>[2x]GGGTPKAPNLEPPLPEEEKEGSDLRPVVIDGSNVAMSHGNKEVF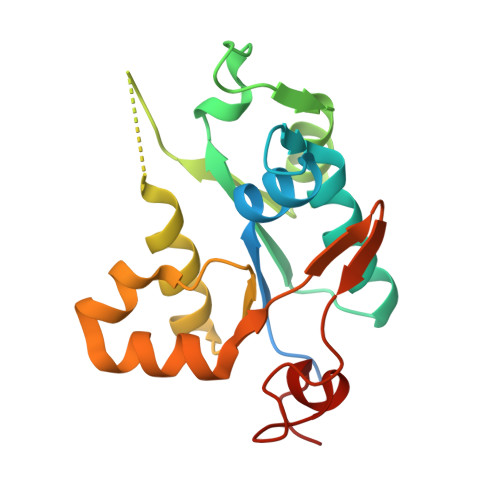SCRGILLAVNWFLERGHTDITVFVPSWRKEQPRPDVPITDQHILRELEKKKILVFTPSRRVGGKRVVCYDDRFIVKLAYESDGIVVSNDTYRDLQGERQEWKRFIEERLLMYSFVNDKFMPPDDPLGRHGPSLDNFLRKKP> ARVAVLISGTGSNLQALIDSTREPNSSAQIDIVISNKAAVAGLDKAERAGIPTRVINHKLYKNRVEFDSAIDLVLEEFSIDIVCLAGFMRILSGPFVQKWNGKMLNIHPSLLPSFKGSNAHEQALETGVTVTGCTVHFVAEDVDAGQIILQEAVPVKRGDTVATLSERVKLAEHKIF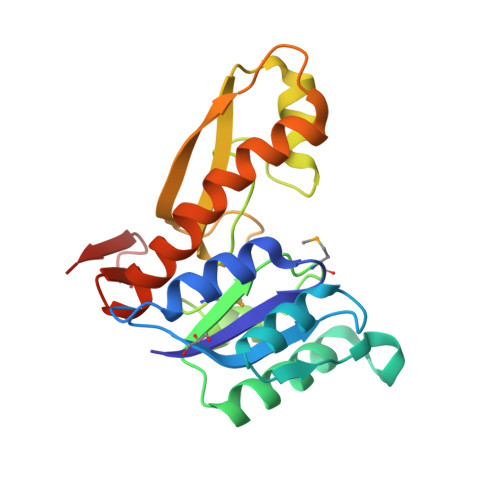PAALQLVASGTVQLGENGKICWVKEE>[2x]AMKLMEVSPLFPCIFLRRVNRFVGLVRIKERIERALITNTGRL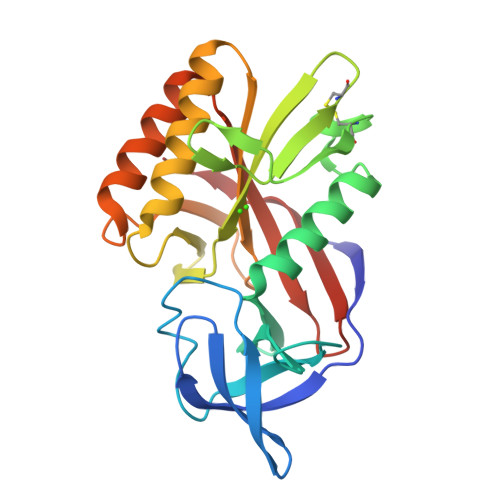NEFMIPGRIGYCTPKAGGKTRYILLGFEDHGKIAIIDTRLQGKAFEKIIEKELLPELEGCRIIKREPRVGESRLDYLIECSKGEIFVETKSAVLREGEYAMYPDCPSVRGQRHIKELIKLARDGKRAMIVFIGALPNVSKFKPYKKGDPKIAELLKEALEAGVEIRALGLHMELSGEIIYRGELGVEI>MRGSHHHHHHGLV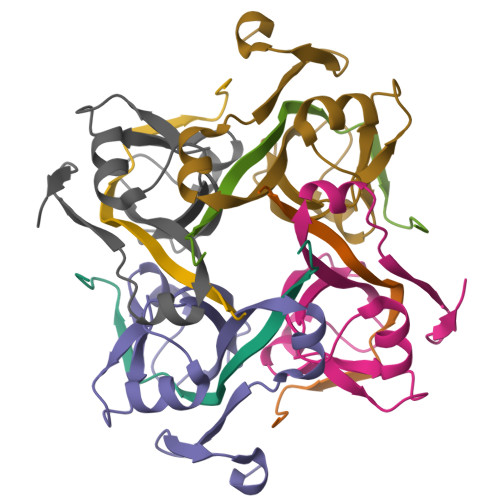PRGSMIRTMLQGKLHRVKVTHADLHYEG[2x];>XCAIDQDFLDAAGILENEAIDIWNVTNGKRFSTYAIAAERGSRIISVNGAAAHCASVGDIVIIASFVTMPDEEARTWRPNVAYFEGDNEMKRTAKAIPVQVA[2x]> MAGNLYGRDGAAIGSLQKLRFFPLAVAGGQGARLVEEDGRELIDLSGAWGAASLGYGHPAIIEAVSRAAANPAGASILSASNAPAVALAERLTASFPGRGTHKVWFGHSGSDANEAAYRAITRATGRTGVIAFIGAYHGCTVGSMAFSGHSVQADAAKADGLILLPYPDPYRPYQDDPTGDAVLALLKERLAAVPAGSIAAAFIEPIQSDGGLIVPPDGFLRKFADICRAHGISVVCDEVKVGLARSGRLHCFEHEGFVPDILVLGKGLGGGLPLSAVIAPAEILDCASAFAMQTLHGNPVCAAAGLAVLETIEAENLTTAAERKGKLLREGLARLAERHELIGDIRGRGLACGVELVRNRQSREPARAETAKLIYRAYELGLVLYYVGMNG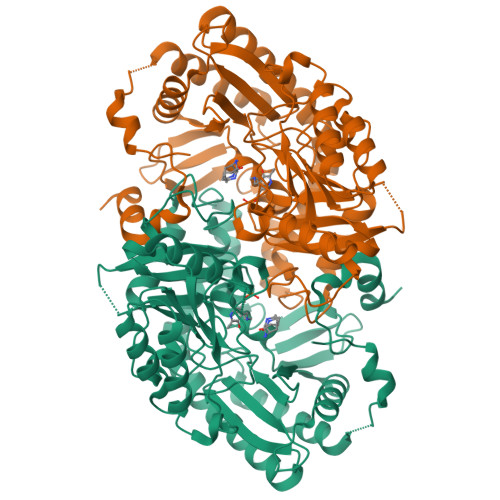NVLEMTPPLTMTEDEVRHAVNLLDQAFTELSTVSDTLVSQFAGW> SISQQTVWNQMATVRTPLNFDSSKQSFCQFSVDLLGGGISVDKTGDWITLVQNSPISNLLRVAAWKKGCLMVKVVMSGNAAVKRSDWASL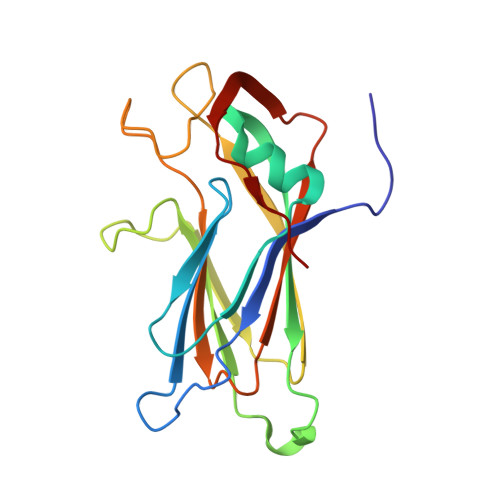VQVFLTNSNSTEHFDACRWTKSEPHSWELIFPIEVCGPNNGFEMWSSEWANQTSWHLSFLVDNPKQSTTFDVLLGISQNFEIAGNTLMPAFSVPQ4-[[(2S)-3-methyl-1-oxo-1-[(2S)-2-[[(3S)-1,1,1-trifluoro-4-methyl-2-oxo-pentan-3-yl]carbamoyl]pyrrolidin-1-yl]butan-2-yl]carbamoyl]benzoic acid | C24 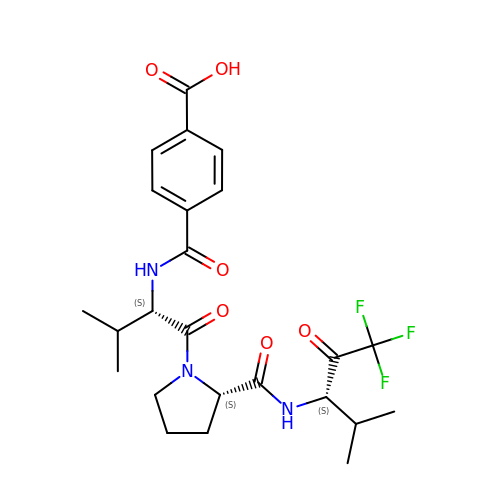H30 F3 N3 O6 | FGNPKLCZJAUKFU-BZSNNMDCSA-N> AVRQRVIPVYQVNNLEEICQLIIQAFEAGVDFQESADSFLLMLCLHHAYQGDYKLFLESGAVKYLEGHGFRFEVKKRDGVKRLEELLPAVSSGKNIKRTLAAMPEEETTEANAGQFLSFASLFLPKLVVGEKACLEKVQRQIQVHAEQGLIQYPTAWQSVGHMMVIFRLMRTNFLIKFLLIHQGMHMVAGHDANDAVISNSVAQARFSGLLIVKTVLDHILQKTERGVRLHPLARTAKVKNEVNSFKAALSSLAKHGEYAPFARLLNLSGVNNLEHGLFPQLSAIALGVATAHGSTLAGVNVGEQYQQLREAATEAE

EBOV is a typical non-segmented negative-sense single-stranded RNA (−ssRNA) virus. Similar to other −ssRNA viruses, the RNA genome of EBOV cannot exist as a naked form, but must be encapsidated by NP and further form a ribonucleoprotein (RNP) complex together with RdRp. Previous studies have demonstrated that N-terminal truncation of EBOV NP resulted the loss-of-function in NP-NP interaction and the first 450 amino-acid of EBOV NP, forming the core domain, is sufficient for the formation of nucleocapsid-like structures and viral genome replication. In particular, this region was revealed to exert the both the function of RNA binding and further NP oligomerization to form high-order RNP.

The best construct with the highest expression yield and biochemical features covers the region of residue 36–351 of EBOV NP (named NPcore hereafter). In the structure of EBOV NPcore, one molecule is observed in the crystallographic asymmetric unit. All residues of EBOV NPcore polypeptide were be built into the final model, except three short gaps (residues A123–S126, E139–T143, K257–R263), and one loop region covering A326–V334 cannot be traced due to the lack of interpretable electron density, indicating their intrinsic structural flexibility. EBOV NPcore is featured by two relatively separate portions, an N-lobe (V36–R240), and a C-lobe (F241–E351). Both two domains are predominantly composed of α-helices, in which the N-lobe consisted of thirteen α-helices and two β-strands and the C-lobe consisted of seven α-helices. The major positive-charged crevice is located in the interface of N-lobe and C-lobe, in which K160, K171, R174, and K248 contribute the most essential positive charge. An additional minor positive-charged region is adjacent to the major crevice and is consisted by R205, K211, and R298. In EBOV NPcore, the hydrophobic pocket is comprised by Helix-14, Helix-15, and Helix-19, a number of hydrophobic residues contributed for the formation of this pocket, including V247, V250, I254, L255, L264, A268, V273, V277, F280, L284, L287, and L316. However, this hydrophobic pocket in occupied by P protein in NiV NP, but is accommodated by Helix-20, which is consisted by residues from N325 to E351, in EBOV NPcore. In the structure of EBOV NPcore alone reported in this work, Helix-20 folds towards and interacts with the hydrophobic pocket on the interface of the C-lobe of EBOV NPcore to form a compact structure.> SESQLKKMVSKYKYRDLTVRETVNVITLYKDLKPVLDSYVFNDGSSR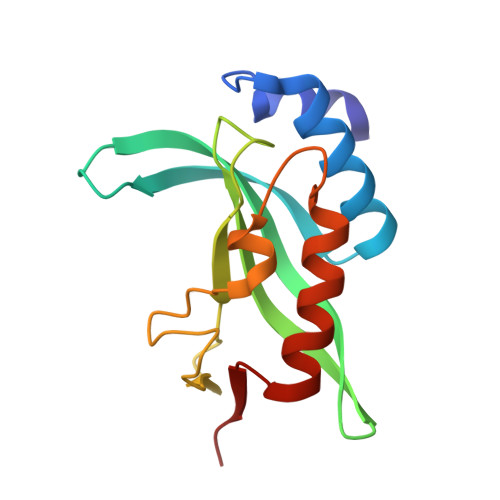ELMNLTGTIPVPYRGNTYNIPICLWLLDTYPYNPPICFVKPTSSMTIKTGKHVDANGKIYLPYLHEWKHPQSDLLGLIQVMIVVFGDEPPVFSRP> MLSVALCFLVGGAIPSPPSFDVTIAPWLIARSRDVLAAPEMLGLRDVLIRSHELSDVEIPLPPGAAVLWRILALITARITGLDQPPNKNPKRKWQARRSQILSKGRLDPEAVDAYFADYSERFDLFHPERPWLQDPRLREECPKTSGVNKLAWGRTAGENQVWLGGHHHDLDPHPLDSAEAVWHLLATLGYGPSGMCTARVVRGRSERNVTAGPLRGTVSYHPLGRTLFESLILNIPYPGTGAADLAFWEQPELNDPLGLPEESAGLAGILRLDHFRHAVLLHPSPDGSHVVDAWVTWAWRERNISPELDPYLIYQTSKEGRVYPRPAEAERAIWRDLDALLHYGEDGNYRPTILDNCTPLAQVPQEVLDSLRLRAFGFDQDGQARDKQWFTATTPAVLRWLADRETDDNENARIVRRITLARKAAEALGRRLEKACKEAWKESNSPSSTS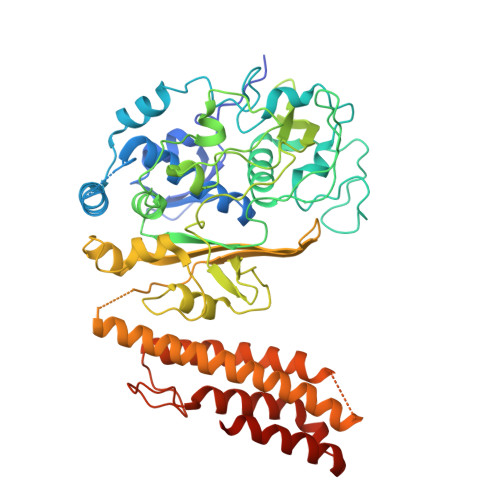SGTNAKTETGVGPWVQHGMSRYWAKAEPVFWNIVYDRPAQGYTPGMAGPGNAFNLVALAAYDEVTGPYCERPRVAKVVERHRSTLFSNWTPKQDKEAA> MSTVVQQVPAELQAALTLINNDPRMRTNNAWALSADKRWSLKFTAELSVPCSSFMPDNSVWHLVLWQEETLIRIEVYPDKSEGISATFQHQNYNFSDASTREWTSGNPALENTP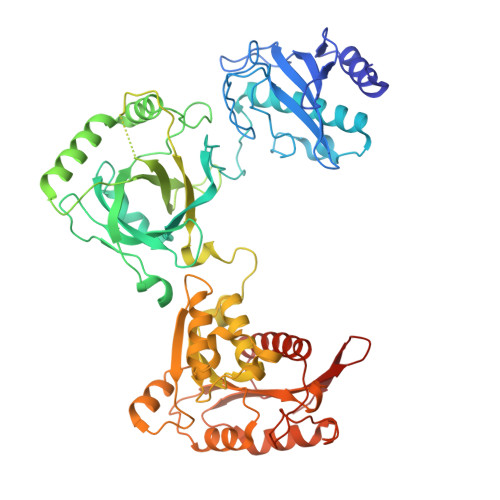TVFGRNLWGLEPEALLDRISWRLSRLLLWIDAAAQEKLATTGDAVELPAFPDQSPFTVIGFSEQIDDLPFWASKTGEWGFASSTGLPGAHGTLFLREFLDNKGKLIRTTKWSPFMRKGARTTNAVWSVLPTLPVLAPWQAPRTWQELSHCFAQCGLSLPDLFSDIGRSVRALRKQRAPGLLLLGFPLENKIGDEPARIHWLALRLAGLSNTMTKRPGFRPTERNRRTWDREQPLSQEPIRWVRTQNWAADQLRTRGEAANDIRSKKVLIIGAGSLGSMIAENLMRIGVVSQGILDADLLQTGNLSRHALTMTSVGHNKAAALVEHLNRILPDASARSFSCAFPPESEVAKNSLRQYDVIIDCTGDDGVLKSLAAFDWKSEKIFISLAMTWRAEGLFAFAASETSFPVTDASSRFNASASPEIDMDEARIEGIGAWHPVFPARADDVQLWAAVGTKFICRVVSAPGRIYEYFKQMPDGTVEKEPHEY>GDICIKDSINTLWTGIKPPPNCQIVENTDTNDGKLTLVLVKNGGLVNGYVSLVGVSDTVNQMFTQKSATIQLRLYFDSSGNLLTDESNLKIPLKNKSSTATSEAATSSKAFMPSTTAYPFNTTTRDSENYIHGICYYMTSYDRSLVPLNISIMLNSRTISSNVAYAIQFEWNLNAKESPESNIATLTTSPFFFSYIREDDN[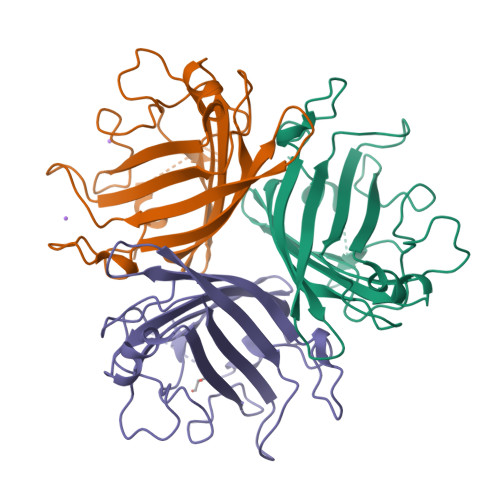12x]> RLSGYCGSPWRVIGYHVVVWMMAGIPLLLFRWKPLWGVRLRLRPCNLAHAETLVIEIRDKEDSSWQLFTVQVQTEAIGEGSLEPSPQSQAEDGRSQAAVGAVPEGAWKDTAQLHKSEEAVSVGQKRVLRYYLFQGQRYIWIETQQAFYQVSLLDHGRSCDDVHRSRHGLSLQDQMVRKAIYGPNVISIPVKSYPQLLVDEALNPYYGFQAFSIALWLADHYYWYALCIFLISSISICLSLYKTRKQSQTLRDMVKLSMRVCVCRPGGEEEWVDSSELVPGDCLVLPQEGGLMPCDAALVAGECMVNESSLTGESIPVLKTALPEGLGPYCAETHRRHTLFCGTLILQARAYVGPHVLAVVTRTGFCTAKGGLVSSILHPRPINFKFYKHSMKFVAALSVLALLGTIYSIFILYRNRVPLNEIVIRALDLVTVVVPPALPAAMTVCTLYAQSRLRRQGIFCIHPLRINLGGKLQLVCFDKTGTLTEDGLDVMGVVPLKGQAFLPLVPEPRRLPVGPLLRALATCHALSRLQDTPVGDPMDLKMVESTGWVLEEEPAADSAFGTQVLAVMRPPLWEPQLQAMEEPPVPVSVLHRFPFSSALQRMSVVVAWPGATQPEAYVKGSPELVAGLCNPETVPTDFAQMLQSYTAAGYRVVALASKPLPTVPSLEAAQQLTRDTVEGDLSLLGLLVMRNLLKPQTTPVIQALRRTRIRAVMVTGDNLQTAVTVARGCGMVAPQEHLIIVHATHPERGQPASLEFLPMESPTAVNGVKDPDQAASYTVEPDPRSRHLALSGPTFGIIVKHFPKLLPKVLVQGTVFARMAPEQKTELVCELQKLQYCVGMCGDGANDCGALKAADVGISLSQAEASVVSPFTSSMASIECVPMVIREGRCSLDTSFSVFKYMALYSLTQFISVLILYTINTNLGDLQFLAIDLVITTTVAVLMSRTGPALVLGRVRPPGALLSVPVLSSLLLQMVLVTGVQLGGYFLTLAQPWFVPLNRTVAAPDNLPNYENTVVFSLSSFQYLILAAAVSKGAPFRRPLYTNVPFLVALALLSSVLVGLVLVPGLLQGPLALRNITDTGFKLLLLGLVTLNFVGAFMLESVLDQCLPACLRRLRPKRASKKRFKQLERELAEQPWPPLPAGPLR

ATP13A2, which is mutated in juvenile-onset Parkinson’s disease and autosomal recessive spastic paraplegia 78, is a transporter with a critical role in balancing the polyamine concentration between the lysosome and the cytosol. The overall structure of hATP13A2 has a canonical P-type ATPase architecture, with the cytosolic A domain linking to TM1 and TM2 domains, and the N and P domains sitting on the TM4 and TM5. The P-type ATPases transport substrates by coupling ATP hydrolysis with protein phosphorylation states and adopting a series of intermediate states, consisting of E1, E1-ATP, E1P-ADP, E1P, E2P, E2-Pi, and E2, in a process known as the Post-Albers reaction. Here, we report seven cryo-EM structures of hATP13A2 in six intermediate states, importantly including the putative E2 and E1-like states, thereby providing a nearly complete atomic-level conformational cycle spanning the Post-Albers reaction process.

Adenine nucleotides (AMP-PCP or ADP) or phosphate analogs (BeF3− or AlF4−) were used to stabilize hATP13A2 in the E1-ATP or E1P/E2P intermediate states. Then, in the following E1P-ADP–to–E2P transition, ADP release from the catalytic center would induce the outward movement of the N-domain by ~25°, which would subsequently alter the architecture of the TM regions, causing entrance pocket Site1 to open toward the luminal side of the lysosome and allowing the recruitment of a polyamine, after which the polyamine would move deeper into Site1 in the subsequent E2-Pi state. Four intermediate states (including E1-ATP, E1P-ADP, E2P, and E2-Pi) were solved at relatively high resolutions (3.2–3.7 Å), whereas the E1-like and putative E2 states were solved at medium resolutions (5.6 Å and 4.8 Å, respectively) probably due to the rapid dynamic equilibrium between the E1 and E2 states.> MAAGQNGHEEWVG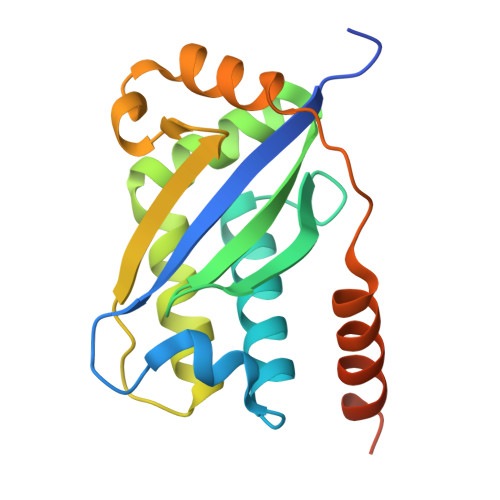SAYLFVESSLDKVVLSDAYAHPQQKVAVYRALQAALAESGGSPDVLQMLKIHRSDPQLIVQLRFCGRQPCGRFLRAYREGALRAALQRSLAAALAQHSVPLQLELRAGAERLDALLADEERCLSCILAQQPDRLRDEELAELEDALRNLKCGSGARGGDGEVASAP> GNYFYNDKQIDVENFYIAELPLTPSQFEEDFKEIHQIVMENYSLYQAKHLNMDSLYQACDARVRQAQTTTDYGLIVQEYISALQCAHAITCYKRYTANQRVAFIEDFLFVDKPNDYLTEYGFQDKDRIIAINGLPYKQWIEQNEKYTEASTVPHRRLRTAYDAFRSYADTLRNYTLLRGGDTLTVTLPLKQRDYFPDNEEQTVESRILQDSIGYLTIKTMMNPVMEDFKAVYPKVKDLPYLIIDVRRNGGGNSMNGVNICKYFIREAQPHCVSKSYIMQPEADAYKGKIYLLTDTYTLSAAESFTLDMKESGNVTLIGEA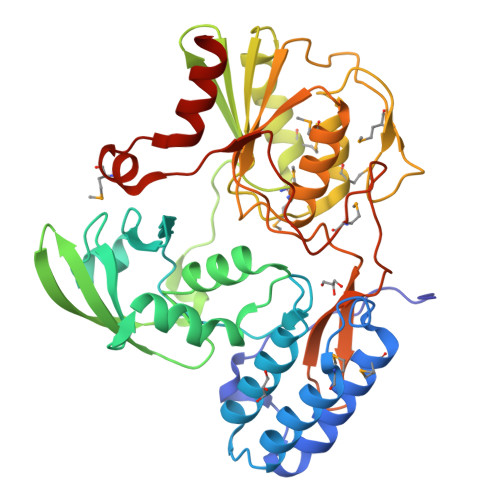TGGDTGNGPRPFCTKQRTYFRIPTRQPDVSSKGFPMEGIGIPPHHQVSQTVADFMKDEDTVLNYAVGLITEKQ> GLIVDTRDVEERVHVMRKTKLAPTVAHGVFNPEFGPAALSNKDPRLNEGVVLDEVIFSKHKGDTKMSAEDKALFRRCAADYASRLHSVLGTANAPLSIYEAIKGVDGLDAMEPDTAPGLPWALQGKRRGALIDFENGTVGPEVEAALKLMEKREYKFACQTFLKDEIRPMEKVRAGKTRIVDVLPVEHI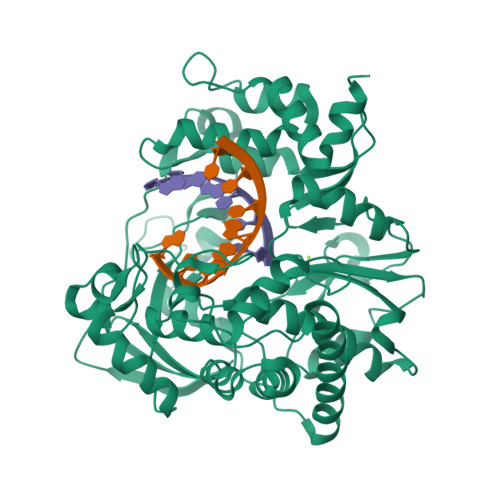LYTRMMIGRFCAQMHSNNGPQIGSAVAANPDVDWQRFGTHFAQYRNVWDVDYSAFDANHCSDAMNIMFEEVFRTEFGFHPNAEWILKTLVNTEHAYENKRITVEGGMPSGCSATSIINTILNNIYVLYALRRHYEGVELDTYTMISYGDDIVVASDYDLDFEALKPHFKSLGQTITPADKSDKGFVLGHSITDVTFLKRHFHMDYGTGFYKPVMASKTLEAILSFARRGTIQEKLISVAGLAVHSGPDEYRRLFEPFQGLFEIPSYRSLYLRWVNAVCGDAAAALEHHHHHH>[2x]GPVWRKHYITYRINNYTPDMNREDVDYAIRKAFQVW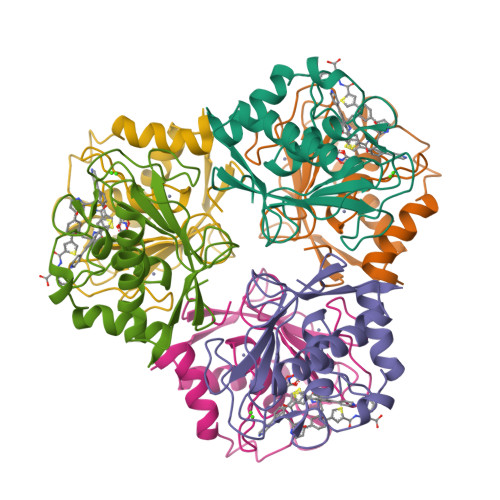SNVTPLKFSKINTGMADILVVFARGAHGDFHAFDGKGGILAHAFGPGSGIGGDAHFDEDEFWTTHSGGTNLFLTAVHEIGHSLGLGHSSDPKAVMFPTYKYVDINTFRLSADDIRGIQSLYGD> EFAITSCPNNETVWETPIGVKYTLCPGSDYQNGGASLQTVRDIQSSLECAKICDSDARCNRAVYDNVNKACDVKNSTNPMQWAADDRFETIRLTNDLPEGAFISTCSFNETSYRVPETNAEYRICPDTDYTGVNAKVVEGVTTIQACAELCSNTQDCRKSVFDHINNACAIKAAEPATSIFWVQDKQFSTIRLPENIDPAVKGKWGDLIRLPVIPVAAYIVPSYPEPSRLLFFSSWSNDAFSGASGMTQFGDYDFATGAISQRTVTNTHHDMFCPGISQLEDGRILIQGGSDADTVSIYDPATNEFTRGPNMTLARGYQTSCTLSNGKVFTIGGAYSGERVGKNGEVYDPVANAWTYLPGADFRPMLTNDHEGIWREDNHAWLFGWKNGSIFQAGPSKDQHWYGIQGNGTVAKAATRDDDDAMCGVWVMYDAVAGKIFSAGGSPDYTDSPATQRAHITTIGEPNTPAEVERVADMGFPRGFANAVVLPDGQVLVTGGQRMSLVFTNTDGILVAELFNPETREWKQMAPMAVPRNYHSVSILLPDATVFSGGGGMCWVQNVGDSTAGCDKTVDHSDGEIFEPPYLFNEDGSRAARPVISAISADPIKAGATLTFTVEGVE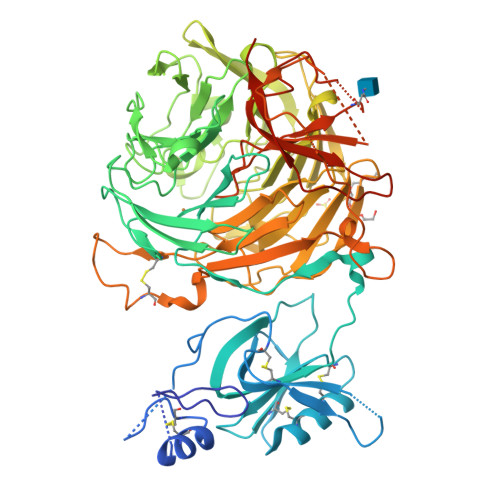GQGTAALIRLGSVTHSVNSDQRRVPLNVTVSGNEYSATLPDDYGILLPGYYYLFVSTPQGTPSIAKTVHVILGLEQKLISEEDLNSAVDHHHHHH DICYCLOHEXYLUREA | C13 H24 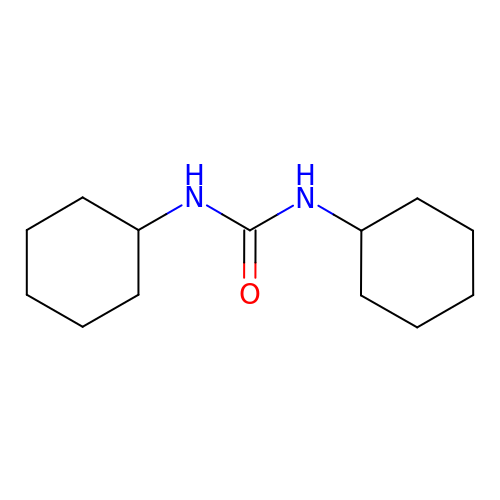N2 O | ADFXKUOMJKEIND-UHFFFAOYSA-N> SPADYTHPTEMRGLSAMDLVKDMKIGWNLGNTLESVGGETGWGNPVTTKKMFDTLKAAGFNTVRIPVRWDENYIDANYTIDPAYMARVETVVNYALANDMYAIVNIHHNKFQGQFDEAHKAAIINEGTIVWTQIANHFKDYSDKLIFDTINQPRHEEDWVGTSEYFNVLNEYNAKIVPVIRATGENNAKRLIMVPTYCA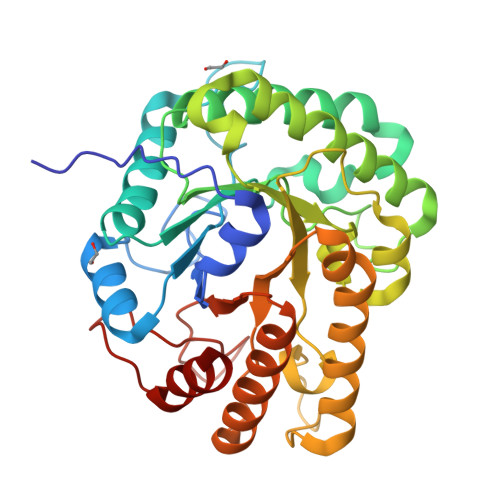SSDYPKVAGMVVPNDPNVAVSIHAYIPYNLALNIAPGTPTTFGDADAAFIDKTFRMLNNTFVKKGIPVIIGQFAITDKDNLQDRINFTKFYVSTATAYGMPCLWWDNNNFGSTGERLGLLNRKNLTFPYPELVQAMKDGFN>AQYEDGKQYTTLEKPVAGAPQVLEFFSFFCPHCYQFAEVLHISDNVKKKLPEGVKMTKYHVNFMGGDLGKDLTQAWAVAMALGVEDKVTVPLFEGVQKTQTIRSASDIRDVFINAGIKGEEYDAAWNSFVVKSLVAQQEKAAADVQLRGVPAMFVNGKYQLNPQGMDTSNMDVFVQQYADTVKYLSEKK[4x]

DsbA from E. coli K−12 (EcDsbA) was the first and is probably the best-characterised DSB enzyme to date. This 21 kDa periplasmic protein is a dithiol oxidase that catalyses disulphide bond formation between consecutive cysteines of unfolded polypeptides as they are translocated to the periplasm. EcDsbA consists of a canonical TRX domain, a hallmark of proteins involved in redox homeostasis, with an inserted helical domain. The TRX domain harbours the conserved active site CXXC (C30-P31-H32-C33 in EcDsbA) that is featured in many proteins of the TRX superfamily. The acidity of this groove originates from a cluster of negatively charged residues (E24, E37, E38, D44, E85, D86 and E94) that map along a buried channel in the interface between the TRX and helical domains of EcDsbA.

The other three mutants, E37A, E24A and E24A/E37A/K58A, were crystallised in space groups P21, P212121 and P2, respectively, with four molecules per asymmetric unit. In this structure, the K58 side chain shifts towards the E24-vacated space, and this change disrupts the proposed salt bridge between K58 and E37. The latter salt bridge was also abolished in the E37A mutant. The hydrogen bond between E37 and water w3 was removed in the E37A mutant structure which has the effect of shortening the distance between w1 and w3 from 3.7 Å in the wildtype structure to 3.3 Å in the mutant structure. Furthermore, the E37A mutation abolished the interaction of E37 with bulk water. Overall, in the E24A and E37A structures, although water molecules w1, w2 and w3 were still present and coordinated to the remaining charged residues in the channel, the number of interactions stabilising these water molecules was reduced, with the E37A mutant also resulting in the water network being less tightly connected to the bulk water (bw1/bw2). E37A caused the most dramatic decrease in the initial rate among single mutants, which was 6-fold slower than that of the wildtype. In agreement with PilQ and ASST peptide oxidation assays, E37A caused the most significant effect among the single mutants, whereby it catalysed PapD peptide oxidation with a rate constant of 1.68 ± 0.12 × 106 M−1 s −1, which is ~26% slower than the wildtype EcDsbA. To investigate whether the water network had been altered upon the introduction of the alanine mutations, we inspected the DsbA alanine mutant crystal structures, which showed that although all point mutants maintained some of the w1–w4 molecules, their position was altered and the tight connectivity of waters to stabilising charged amino acids was considerably reduced. This was especially the case for E37A, which lacked the negatively charged side chain stabilising the buried water network and connecting it with the bulk solvent, which could contribute to initiation of the proton relay. We also found that this mutant showed the lowest oxidase activity of all the single mutants we analysed.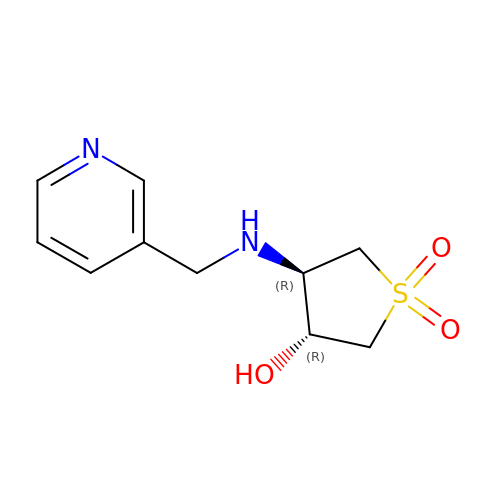(3~{R},4~{R})-1,1-bis(oxidanylidene)-4-(pyridin-3-ylmethylamino)thiolan-3-ol | C10 H14 N2 O3 S | HNCRLYXMUJVCNN-UWVGGRQHSA-N> MLGDVERFFSKKALEMRASEVRELLK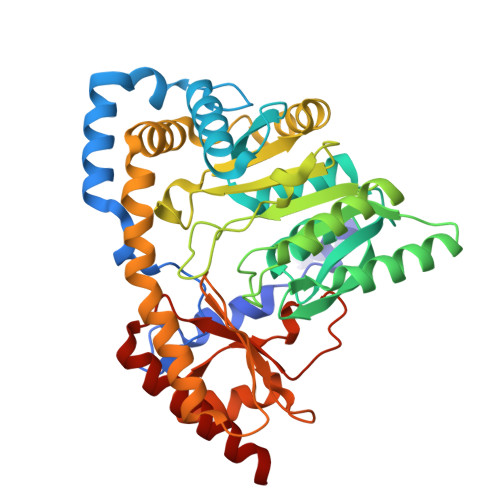LVETSDIISLAGGLPNPKTFPKEIIRDILVEIMEKYADKALQYGTTKGFTPLRETLMKWLGKRYGISQDNDIMITSGSQQALDLIGRVFLNPGDIVVVEAPTYLAALQAFNFYEPQYIQIPLDDEGMKVEILEEKLKELKSQGKKVKVVYTVPTFQNPAGVTMNEDRRKYLLELASEYDFIVVEDDPYGELRYSGNPEKKIKALDNEGRVIYLGTFSKILAPGFRIGWMVGDPGIIRKMEIAKQSTDLCTNVFGQVVAWRYVDGGYLEKHIPEIRKFYKPRRDAMLEALEEFMPEGVKWTKPEGGMFIWVTLPDGIDSKKMLERAIKKGVAYVPGEAFYAHRDVKNTMRLNFTYVDEDKIMEGIKRLAETIKEELKA>[5x]MSIAVNMNDPTNTGVKTTTGSGSMTGSNAADLQSSFLTLLVAQLKNQDPTNPLQNNELTTQLAQISTVSGIEKLNTTLGAISGQIDNSQSLQATTLIGHGVMVPGTTILAGKGAEEG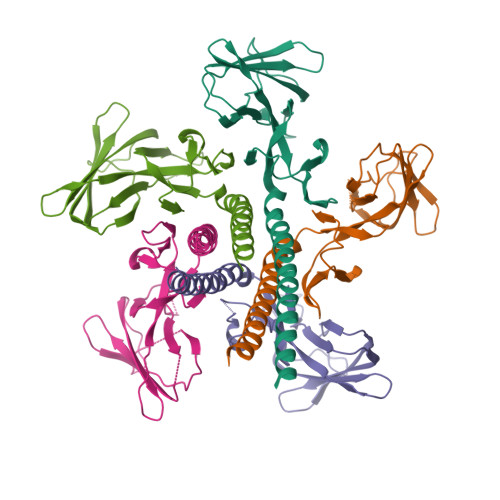AVTSTTPFGVELQQPADKVTATITDKDGRVVRTLEIGELRAGVHTFTWDGKQTDGTTVPNGSYNIAITASNGGTQLVAQPLQFALVQGVTKGSNGNLLDLGTYGTTTLDEVRQII>[4x]MGYHLGATFPNFTAKASGIDGDFELYKYIENSWAILFSHPNDFTPVCTTEL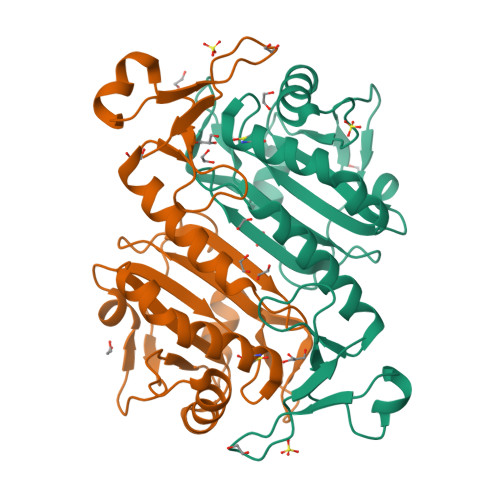AELGKMHEDFLKLNCKLIGFSCNSKESHDKWIEDIKYYGKLNKWEIPIVCDESRELANKLKIMDEQEKDITGLPLTCRCLFFISPEKKIKATVLYPATTGRNAHEILRVLKSLQLTYTTPVATPVNWNEGDKCCVIPTLQDDEISKHFKNEITKVEMPSKKKYLRFVNL>MPSEAKYTWDQELNEINIQFPVTGD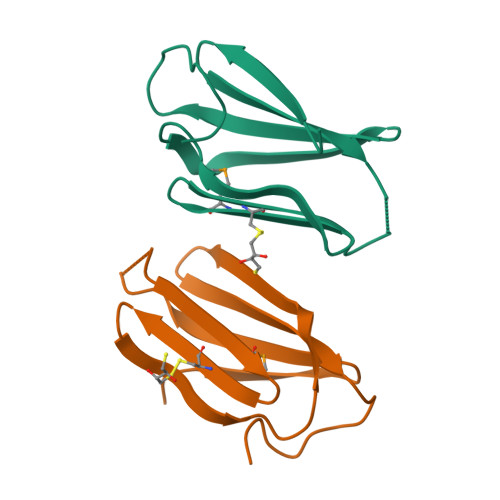ADSSAIKIRMVGKKICVKNQGEIVIDGELLHEVDVSSLWWVINGDVVDVNVTKKRNEWWDSLLVGSESVDVQKLAENKHADMSMLDAEAREVVEKMMHNTSGKDSE[2x]>SNAMIDFACKEFKVEDVIKCALNLTKADLNVMKSFLNEPDRWIDTDALSKSLKLDVSTVQRSVKKL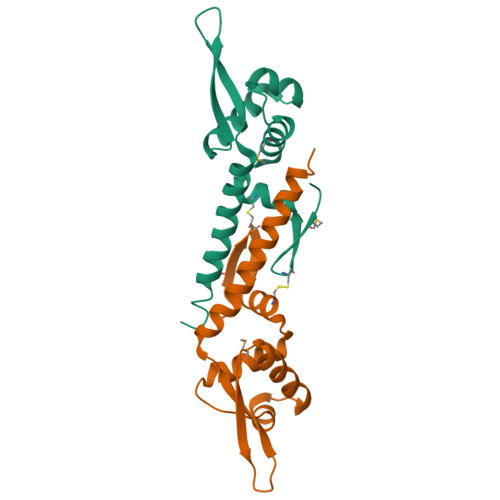HEKEILQRSQQNLDGGGYVYIYKIYSKNQIRNIIQKIVQSWADRLGQELKEWENGGE[2x]> MLEQPYLDLAKKVLDEGHFKPDRTHTGTYSIFGHQMRFDLSKGFPLLTTKKVPFGLIKSELLWFLHG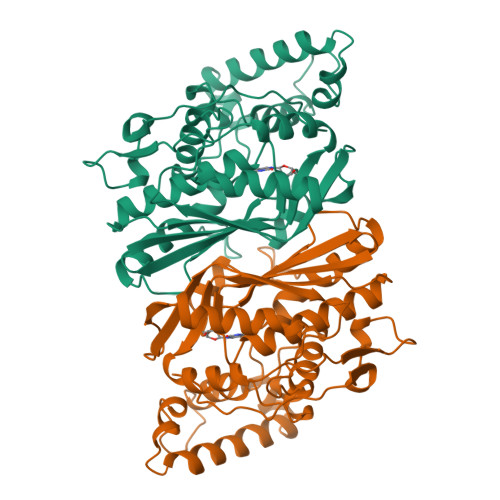DTNIRFLLQHRNHIWDEWAFEKWVKSDEYHGPDMTDFGHRSQKDPEFAAVYHEEMAKFDDRVLHDDAFAAKYGDLGLVYGSQWRAWHTSKGDTIDQLGDVIEQIKTHPYSRRLIVSAWNPEDVPTMALPPCHTLYQFYVNDGKLSLQLYQRSADIFLGVPFAIASYALLTHLVAHECGLEVGEFIHTFGDAHLYVNHLDQIKEQLSRTPRPAPTLQLNPDKHDIFDFDMKDIKLLNYDPYPAIKAPVAV>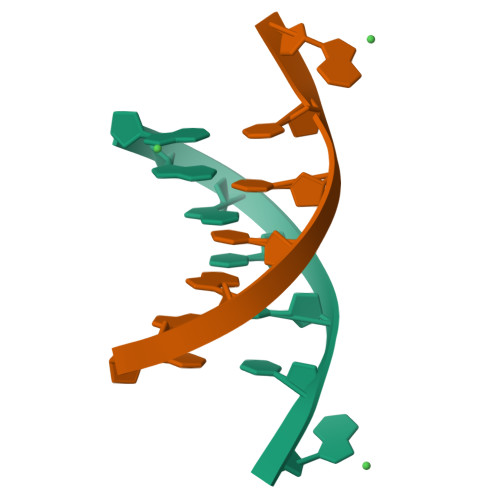[2x]GAATTCG> LAAGTPALGDDRGRPWPASLAALALDGKLRTDSNATAAASTDFGNITSALPAAVLYPSSTADLVALLSAANSTPGWPYTIAFRGRGHSLMGQAFAPGGVVVNMASLGDAAAPPRINVSADGRYVDAGGEQVWIDVLRASLARGVAPRSWTDYLYLTVGGTLSNAGISGQAFRHGPQISNVLEMDVITGHGEMVTCSKQLNADLFDAVLGGLGQFGVITRARIAVEPAPARARWVRLVYTDFAAFSADQERLTAPRPGGGGASFGPMSYVEGSVFVNQSLATDLANTGFFTDADVARIVALAGERNATTVYSIEATLNYDNATAAAAAVDQELASVLGTLSYVEGFAFQRDVAYAAFLDRVHGEEVALNKLGLWRVPHPWLNMFVPRSRIADFDRGVFKGILQGTDIVGPLIVYPLNKSMWDDGMSAATPSEDVFYAVSLLFSSVAPNDLARLQEQNRRI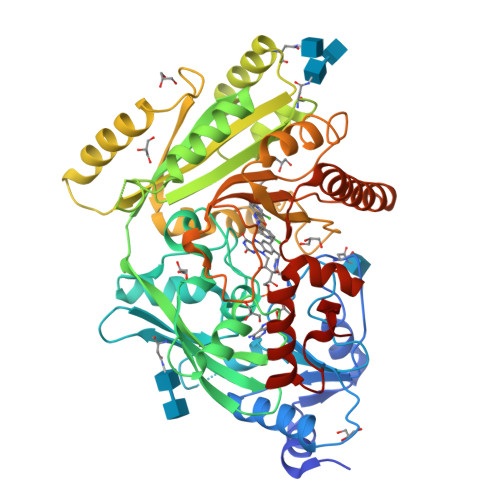LRFCDLAGIQYKTYAARHTDRSDWVRHFGAAKWNRFVEMKNKYDPKRLLSPGQDIFN> GPLGSMMPEINTNHLDKQQVQLLAEMCILIDENDNKIGAET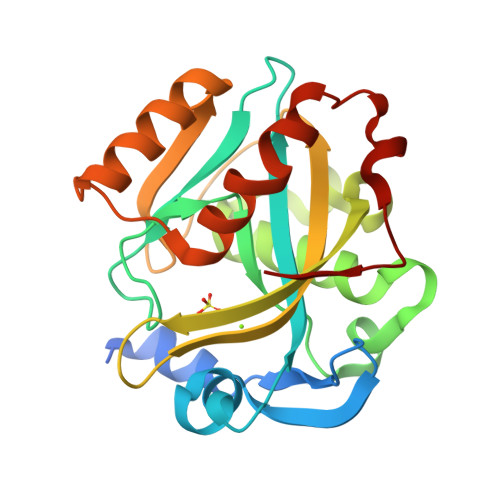KKNCHLNENIEKGLLHRAFSVFLFNTENKLLLQQRSDAKITFPGCFTNTCCSHPLSNPAELEESDALGVRRAAQRRLKAELGIPLEEVPPEEINYLTRIHYKAQSDGIWGEHEIDYILLVRKNVTLNPDPNEIKSYCYVSKEELKELLKKAASGEIKITPWFKIIAATFLFKWWDNLNHLNQFVDHEKIYRM N1-((2S,3S,5R)-3-AMINO-6-(4-FLUOROPHENYLAMINO)-5-METHYL-6-OXO-1-PHENYLHEXAN-2-YL)-N3,N3-DIPROPYLISOPHTHALAMIDE 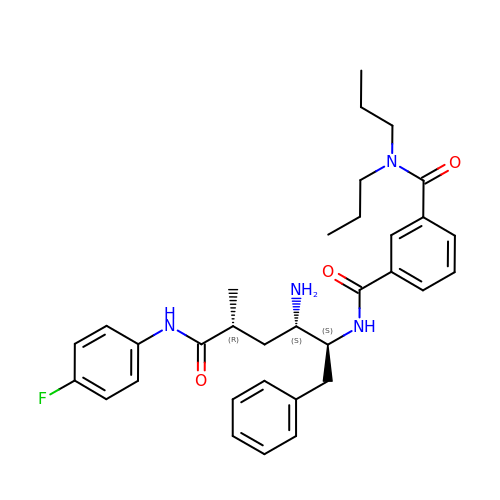| C33 H41 F N4 O3 | PZHFCAIXAVDQAK-STQWGSIPSA-N>[3x]MDFSKLPKIRDEDKESTFGYVHGVSGPVVTACDMAGAAMYELVRVGHSELVGEIIRLEGDMATIQVYEETSGVSVGDPVLRTGKPLSVELGPGIMGAIFDGIQRPLSDISSQTQSIYIPRGVNVSALSRDIKWEFIPSKNLRVGSHITGGDIYGIVNENSLIKHKIMLPPRSRGSVTYIAPPGNYDASDVVLELEFEGVKEKLSMVQVWPVRQVRPVTEKLPANHPLLTGQRVLDALFPCVQGGTTAIPGAFGCGKTVISQSLSKYSNSDVIIYVGCGERGNEMSEVLRDFPELTMEVDGKVESIMKRTALVANTSNMPVAAREASIYTGITLSEYFRDMGYHVSMMADSTSRWAEALREISGRLAEMPADSGYPAYLGARLASFYERAGRVKCLGNPEREGSVSIVGAVSPPGGDFSDPVTSATLGIVQVFWGLDKKLAQRKHFPSVNWLISYSKYMRALDEYYDKHFTEFVPLRTKAKEILQEEEDLAEIVQLVGKASLAETDKITLEVAKLIKDDFLQQNGYTPYDRFCPFYKTVGMLSNMISFYDMARRAVETTAQSDNKITWSIIREHMGEILYKLSSMKFKDPVKDGEAKIKADYAQLLEDMQNAFRSLED;>MALRAMRGIVNGAAPELPVPTGGPMAGAREQALAVSRNYLSQPRLTYKTVSGVNGPLVILDHVKFPRYAEIVHLTLPDGTKRSGQVLEVSGSKAVVQVFEGTSGIDAKKTSCEFTGDILRTPVSEDMLGRVFNGSGKPIDRGPVVLAEDFLDIMGQPINPQCRIYPEEMIQTGISAIDGMNSIARGQKIPIFSAAGLPHNEIAAQICRQAGLVKKSKDVVDYSEENFAIVFAAMGVNMETARFFKSDFEENGSMDNVCLFLNLANDPTIERIITPRLALTTAEFLAYQCEKHVLVILTDMSSYAEALREVSAAREEVPGRRGFPGYMYTDLATIYERAGRVEGRNGSITQIPILTMPNDDITHPIPDLTGYITEGQIYVDRQLHNRQIYPPINVLPSLSRLMKSAIGEGMTRKDHADVSNQLYACYAIGKDVQAMKAVVGEEALTSDDLLYLEFLQKFEKNFITQGPYENRTVYETLDIGWQLLRIFPKEMLKRIPQSTLSEFYPRDSAKH[3x];> MSGKDRIEIFPSRMAQTIMKARLKGAQTGRNLLKKKSDALTLRFRQILKKIIETKMLMGEVMREAAFSLAEAKFTAGDFSTTVIQNVNKAQVKIRAKKDNVAGVTLPVFEHYHEGTDSYELTGLARGGEQLAKLKRNYAKAVELLVELASLQTSFVTLDEAIKITNRRVNAIEHVIIPRIERTLAYIITELDEREREEFYRLKKIQEKKKIIKEKSEKDLERRRAAGEVMEPANLLAEEKDEDLLFE;>[3x]MALSDADVQKQIKHMMAFIEQEANEKAEEIDAKAEEEFNIEKGRLVQTQRLKIMEYYEKKEKQIEQQKKIQMSNLMNQARLKVLRARDDLITDLLNEAKQRLSKVVKDTTRYQVLLDGLVLQGLY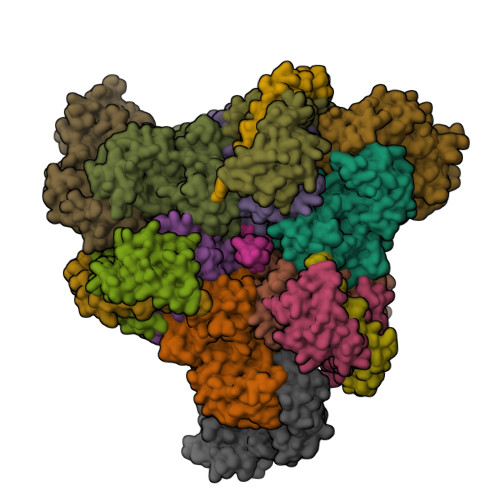QLLEPRMIVRCRKQDFPLVKAAVQKAIPMYKIATKKDVDVQIDLEAYLPEDIAGGVEIYNGDRKIKVSNTLESRLDLIAQQMMPEVRGALFGANANRKFLD;>MASQSQGIQQLLQAEKRAAEKVADARKRKARRLKQAKEEAQMEVEQYRREREQEFQSKQQAAMGSQGNLSAEVEQATRRQVQGMQSSQQRNRERVLTQLLGMVCDVRPQVHPNYRITV[3x];>[3x]GMSFIKVGIKMGGLTSEQYHSQVVGKIGYIARCMQTIDPENNLKKIREDYQDVLIWAEKNYRFEEILEASKSGKCPNDLDALSRRSLILQELLRLVSSISPFKMKLDLIESQYEKMKQHVNLWKSDYHVKLNQLNQLTDYLKNAAPTPKNNFLRAMTSVLQMQIAQYGITEDNEGINQLFKLGLHLLAMANEKIDEQYHLFKGYVKDQPEESPFEGILPAEDQKILVKTMIDYAMPKLSSKVLQDKLSALSSSDVLTKTLLDSIDRIVKENEKLNALSKDYKDHDGDYKDHDIDYKDDDDK> GNKSEDKLSGDDFWAQGNETNAEAFLLSIYNSFRNATMSQRPFLTYSGDMRCAPITAYSTGDKYVAYLANNDMGELRNTYPDDARGGLIMQWDVFYTA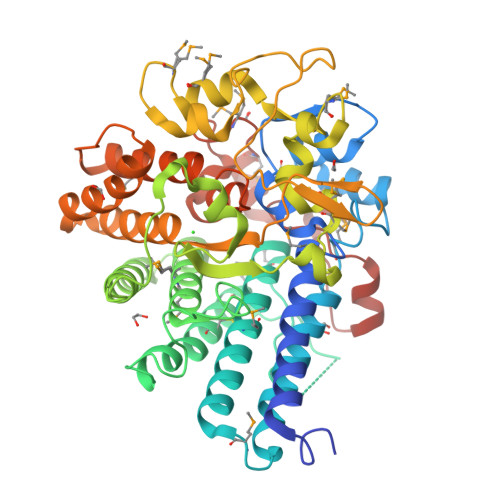IQDANILLAEIDKVPGMDELKRSRFKAEAIFMRSLSYFFIVRAFGDVPYYTNAYNEAPLPRTNMVIVLQNCLADLQPLLDDDPGAEVLPWSYSSYSSKGIRASRGSVIALMMHINLWLVQFDAQNKEQYYRNVVSLGEELERNNGAYSLLDINRSSVIFAGGSDEGLFEIAQNINFNEIFMMNAKFSDNVSYSCLNKSMPLFCYSGDYLMTLFPMYEDDARKELWFDEKIYSTSVSSSAPKEIKKFWNIDTYGNGTITSNSGNQIVFRYAGALLLYAEALAALGTNDTKACELLNRVRNRAHASEINTSGSELMDAIFWERCRELIGEGHYYYDLVRTGKVYNRNYCMNPMTRTNFNVGAWTWPIHRNALKNNTQIGLNLFWE> MTVFRQENVDDYYDTGEELGSGQFAVVKKCREKSTGLQYAAKFIKKRRTKSSRRGVSREDIEREVSILKEIQHPNVITLHEVYENKTDVILILELVAGGELFDFLAEKESLTEEEATEFLKQILNGVYYLHSLQIAHFDLKPENIMLLDRNVPKPRIKIIDFGLAHKIDFGNEFKNIFGTPEFVAPEIVNYEPLGLEADMWSIGVITYILLSGASPFLGDTKQETLANVSAVNYEFEDEYFSN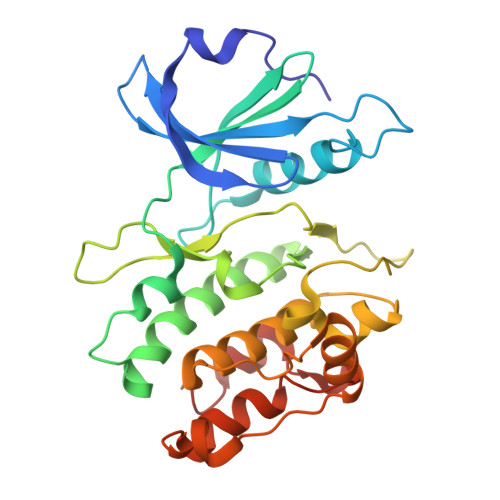TSALAKDFIRRLLVKDPKKRMTIQDSLQHPWIKPK2-[4-(4-cyano-3-methylphenoxy)phenyl]-N-ethyl-N-[2-(1H-pyrazol-1-yl)ethyl]acetamide | C23 H24 N4 O2 | 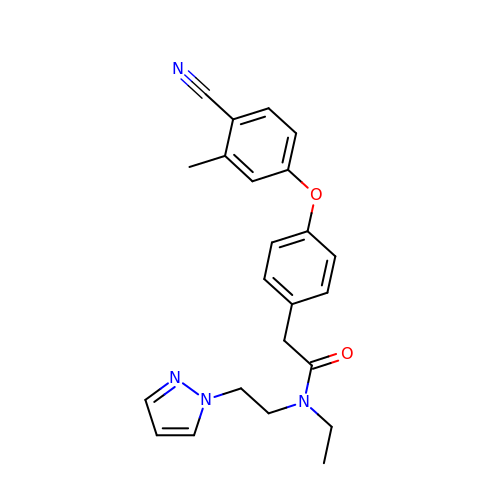ABKHTUJKHPJZLS-UHFFFAOYSA-N>[2x]MMEYKIVENGLTYRIGNGASVPISNTGELIKGLRNYGPYEVPSLKYNQIALIHNNQFSSLINQLKSQISSKIDEVWHIHNINISEFIYDSPHFDSIKSQV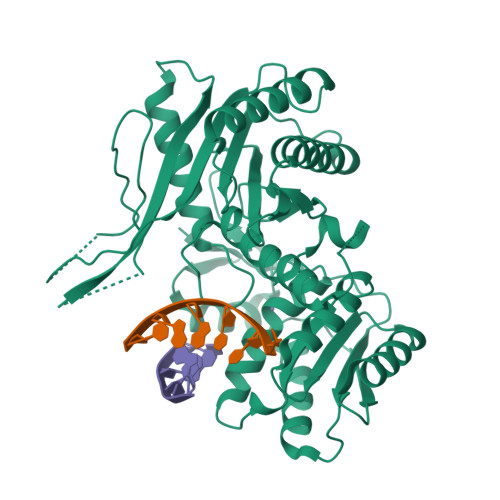DNAIDTGVDGIMLVLPEYNTPLYYKLKSYLINSIPSQFMRYDILSNRNLTFYVDNLLVQFVSKLGGKPWILNVDPEKGSDIIIGTGATRIDNVNLFCFAMVFKKDGTMLWNEISPIVTSSEYLTYLKSTIKKVVYGFKKSNPDWDVEKLTLHVSGKRPKMKDGETKILKETVEELKKQEMVSRDVKYAILHLNETHPFWVMGDPNNRFHPYEGTKVKLSSKRYLLTLLQPYLKRNGLEMVTPIKPLSVEIVSDNWTSEEYYHNVHEILDEIYYLSKMNWRGFRSRNLPVTVNYPKLVAGIIANVNRYGGYPINPEGNRSLQTNPWFL>[12x]GPHMRLEECRKRLEELEAAREELLKVLREMRIHSTKSI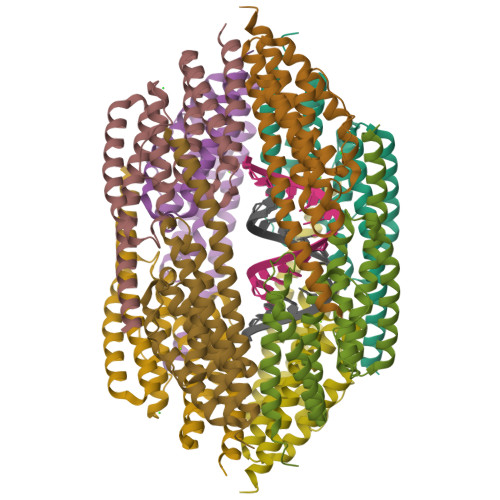ALIHAGKVEEAEQELKKAIELLEKVKAYREYPEIYFYLCNDAMQELVEAIAFKNAISGEFTFEIDLEVTPAAFLNGFAAAVGELRRYALTKLIEGDFKSAERMLEVMEKIYERLMEFTTFPDKLVSGLRKKLDVARGGIERTKSDYIAAKVARLNESLGGN> MSQDNREIVMKYISYKLSQRGYEWDAGDVEENRT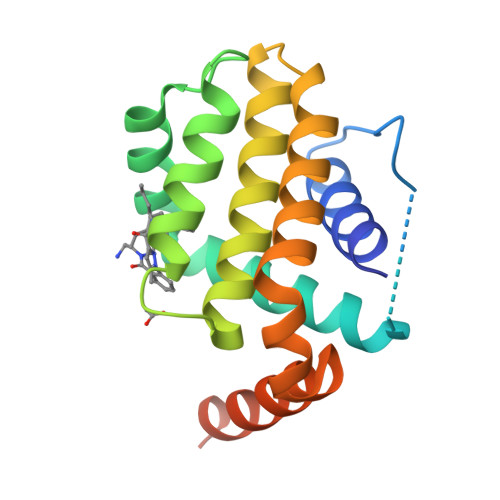EAPEGTESEVVHQTLRQAGDDFSLRYRRDFAQMSSQLHLTPGTAYASFATVVAELFRDGVNWGRIVAFFEFGGVMCVESVNRAMSVLVDNIAAWMATYLNDHLHTWIQDNGGWDAFVELYGNNAAAESRKGQERFLEHHHHHH>SPEVTMNISQMITYWGYPNEEYEVVTEDGYILEVNRIPYGKKNSGNTGQRPVVFLQHGLLASATNWISNLPNNSLAFILADAGYDVWLGNSRGNTWARRNLYYSPDSVEFWAFSFDEMAKYDLPATIDFIVKKTGQKQLHYVGHSQGTTIGFIAFSTNPSLAKRIKTFYALAPVATVKYTKSLINKLRFVPQSLFKFIFGDKIFYPHNFFDQFLATEVCSREMLNLLCSNALFIICGFDSKNFNTSRLDVYLSHNPAGTSVQNMFHWTQAVKSGKF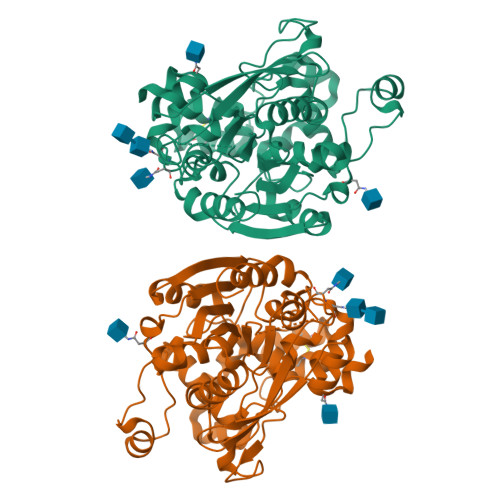QAYDWGSPVQNRMHYDQSQPPYYNVTAMNVPIAVWNGGKDLLADPQDVGLLLPKLPNLIYHKEIPFYNHLDFIWAMDAPQEVYNDIVSMISEDKK[2x]>MVTAHFVLIHTICHGAWIWHKLKPALER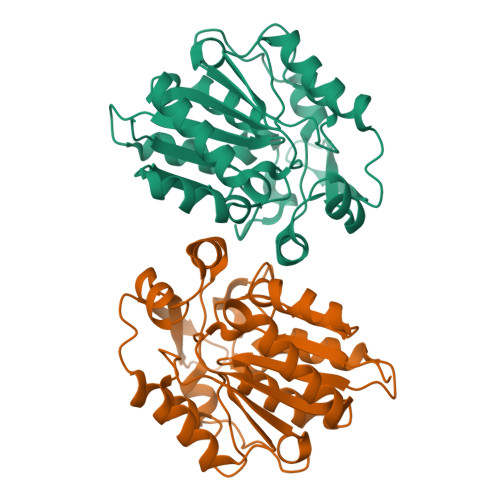AGHKVTALDMAASGIDPRQIEQINSFDEYSEPLLTFLESLPQGEKVIIVGESCAGLNIAIAADKYVDKIAAGVFHNSLLPDTVHSPSYVVEKLLESFPDWRDTEYFTYTNNTGETITTMKLGFKLLRENLYTKCTDEEYELAKMVMRKGSLFQNVLAQRPKFTEKGYGSIKKVYIWTDQDKIFLPDFQRWQIANYKPDKVYQVQGGDHKLQLTKTEEVAHILQEVADAYALEHHHHHH[4x]> GDRVADVIESSIGDSVSRALTHALPAPTGQNTQVSSHRLDTGKVPALQAAEI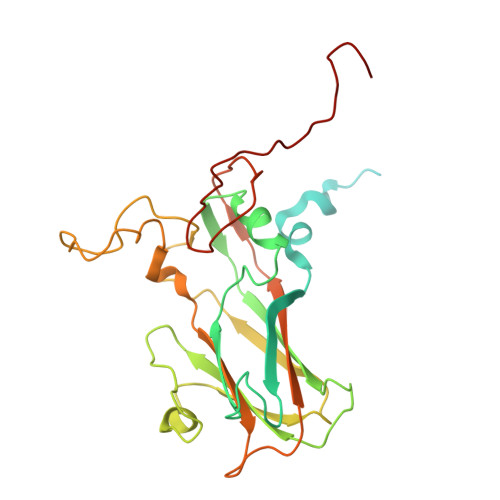GASSNASDESMIETRCVLNSHSTAETTLDSFFSRAGLVGEIDLPLEGTTNPNGYANWDIDITGYAQMRRKVELFTYMRFDAEFTFVACTPTGEVVPQLLQYMFVPPGAPKPDSRESLAWQTATNPSVFVKLSDPPAQVSVPFMSPASAYQWFYDGYPTFGEHLQANDLDYGACPNNMMGTFSVRTVGTSKSKYPLVVRIYMRMKHVRAWIPRPMRNQNYLFKANPNYAGNSIKPTGASRTAITTL> SRVLLALHDRAPQLKISDDRLTVVGEKGYSMVRASHGVRKGAWYFEITVDEMPPDTAARLGWSQPLGNLQAPLGYDKFSYSWRSKKGTKFHQSIGKHYSSGYGQGDVLGFYINLPEDTISGRGSSEIIFYKNGVNQGVAYKDIFEGVYFPAISLYKSCTVSINFGPCFKYPPKDLTYRPMSDMG;> SDLPMPMRFRHLKKTSKEAVGVYRSPIHGRGLFCKRNIDAGEMVIEYAGIVIRSILTDKREKYYDSKGIGSSYMFRIDDSEVVDATMHGNAARFINHSCEPNCYSRVINIDGQKHIVIFAMRKIYRGEELTYDYKFP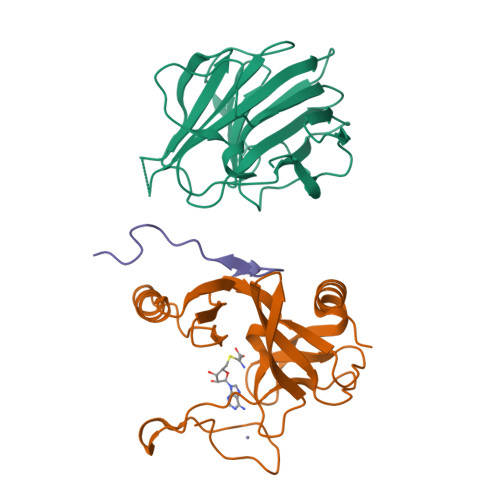IEDASNKLPCNCGAKKCRKFLN;> SAFAPDFKELDENVEYEERESEFDIED> HHHHHHHHHHENLYFQSHMSAKKIVLKSSDGESFEVEEAVALESQ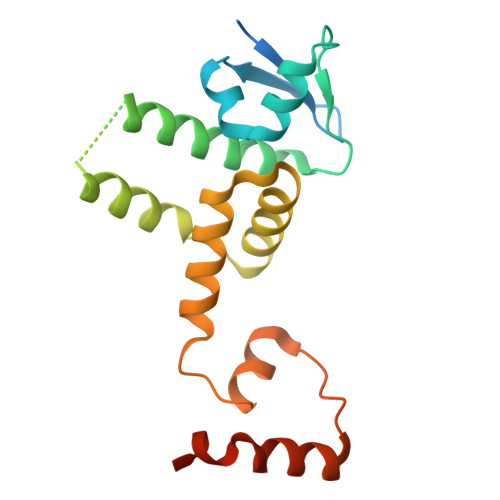TIAHMVEDDCVDNGVPLPNVTSKILAKVIEYCKRHVEAAASKAEAVEGAATSDDDLKAWDADFMKIDQATLFELILAANYLNIKNLLDLTCQTVADMIKGKTPEEIRTTFNIKNDFTPEEEEEVRRENQWAFEGGYKDDDDK To achieve colonization of the stomach, this Gram-negative bacterium adheres to Lewisb (Leb) antigens in the gastric mucosa using its outer membrane protein BabA. The blood group antigen–binding adhesin (BabA) is one of the best-characterized adhesion proteins of the bacterium. It contains two domains: an N-terminal extracellular host-binding domain (7–9) and a C-terminal outer membrane–spanning domain predicted to form a β-barrel structure similar to that of known porins. BabA is a predominantly α-helical molecule with a markedly kinked tertiary structure containing a single, shallow Leb binding site at its tip within a β-strand motif.

We first determined the crystal structure of the N-terminal extracellular domain of BabA, from strain J99 (19), to 2.0-Å resolution. BabA contains two predominantly α-helical regions—a handle and head region, and a third β-sheet motif located on top of the head region. We term this β-strand unit the crown. The handle region, containing both the N and C termini of the extracellular domain, forms an α+β unit. The N-terminal helix (α-N) forms a two-helix antiparallel coiled-coil bundle with a C-terminal helix (α-C1) of similar approximate length. The core of the head region is composed of a four-helix antiparallel coiled-coil bundle, similar to a tetratricopeptide repeat motif (α-1 to α-4), at a near perpendicular angle to the handle region creating the markedly kinked tertiary structure. The connecting features between these four helices are (i) a loop containing a short α-helix (followed by a disordered region of seven amino acids) between α-3 and α-4; (ii) a 20–amino acid loop between α-2 and α-3; and (iii) a ~200–amino acid segment (including a disordered region of 8 amino acids) between the α-1 and α-2 helices. This connecting segment, which extends out of the core of the head region, contains a small β-sheet (β-1), a pair of interacting α-helices (α-1a and α-1b), and the crown—a four-strand antiparallel β-sheet at the highest tip of the protein (β-2). BabA belongs to the Helicobacter outer membrane porins (Hop) family, from which the crystal structure of the functionally related sialic acid–binding adhesin (SabA), from H. pylori strain 26695, has been determined. Whereas both proteins share highly similar three-dimensional folds, the four-strand antiparallel β-sheet crown of BabA is altogether absent in SabA.

> GYQIGEAAQMVTNTKGIQDLSDRYESLNNLLNRYSTLNTLIKLSADPSAINAVRENLGASAKNLIGDKANSPAYQAVLLAINAAVGFWNVVGYVTQCGGNANGQKSISSKTIFNNEPGYRSTSITCSLNGHSPGYYGPMSIENFKKLNEAYQILQTALKRGLPALKENNGKVNVTYTYTCSGDGNNNCSSQVTGVNNQKDGTKTKIQTIDGKSVTTTISSKVVDSRADGNTTGVSYTEITNKLEGVPDSAQALLAQASTLINTINNACPYFHASNSSEANAPKFSTTTGKICGAFSEEISAIQKMITDAQELVNQTSVINEHEQTTPVGNNNGKPFNPFTDASFAQGMLANASAQAKMLNLAEQVGQAINPERLSGTFQNFVKGFLATCNNPSTAGTGGTQGSAPGTVTTQTFASGCAYVGQTITNLKNSIAHFGTQEQQIQQAENIADTLVNFKSRYSELGNTYNSITTALSNIPNAQSLQNAVSKKNNPYSPQGIDTNYYLNQNSYNQIQTINQELKKKKKKGSEQKLISEEDLSHHHHHH> MLHLSAAPPAPPPEVTATARPCLCSVGRRGDGGKMAAAGALERSFVELSGAERERPRHFREFTVCSIGTANAVAGAVKYSESAGGFYYVESGKLFSVTRNRFIHWKTSGDTLELMEESLDINLLNNAIRLKFQNCSVLPGGVYVSETQNRVIILMLTNQTVHRLLLPHPSRMYRSELVVDSQMQSIFTDIGKVDFTDPCNYQLIPAVPGISPNSTASTAWLSSDGEALFALPCASGGIFVLKLPPYDIPGMVSVVELKQSSVMQRLLTGWMPTAIRGDQSPSDRPLSLAVHCVEHDAFIFALCQDHKLRMWSYKEQMCLMVADMLEYVPVKKDLRLTAGTGHKLRLAYSPTMGLYLGIYMHAPKRGQFCIFQLVSTESNRYSLDHISSLFTSQETLIDFALTSTDIWALWHDAENQTVVKYINFEHNVAGQWNPVFMQPLPEEEIVIRDDQDPREMYLQSLFTPGQFTNEALCKALQIFCRGTERNLDLSWSELKKEVTLAVENELQGSVTEYEFSQEEFRNLQQEFWCKFYACCLQYQEALSHPLALHLNPHTNMVCLLKKGYLSFLIPSSLVDHLYLLPYENLLTEDETTISDDVDIARDVICLIKCLRLIEESVTVDMSVIMEMSCYNLQSPEKAAEQILEDMITIDVENVMEDICSKLQEIRNPIHAIGLLIREMDYETEVEMEKGFNPAQPLNIRMNLTQLYGSNTAGYIVCRGVHKIASTRFLICRDLLILQQLLMRLGDAVIWGTGQLFQAQQDLLHRTAPLLLSYYLIKWGSECLATDVPLDTLESNLQHLSVLELTDSGALMANRFVSSPQTIVELFFQEVARKHIISHLFSQ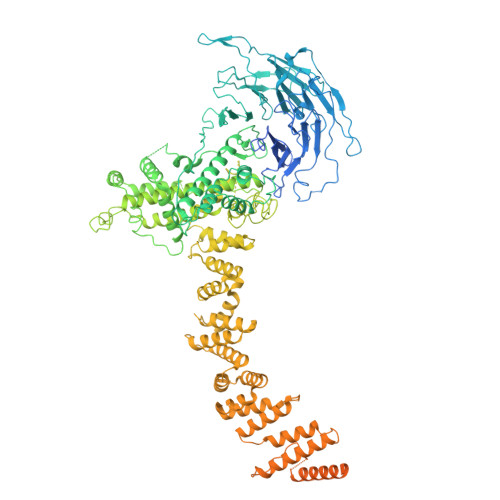PKAPLSQTGLNWPEMITAITSYLLQLLWPSNPGCLFLECLMGNCQYVQLQDYIQLLHPWCQVNVGSCRFMLGRCYLVTGEGQKALECFCQAASEVGKEEFLDRLIRSEDGEIVSTPRLQYYDKVLRLLDVIGLPELVIQLATSAITEAGDDWKSQATLRTCIFKHHLDLGHNSQAYEALTQIPDSSRQLDCLRQLVVVLCERSQLQDLVEFPYVNLHNEVVGIIESRARAVDLMTHNYYELLYAFHIYRHNYRKAGTVMFEYGMRLGREVRTLRGLEKQGNCYLAALNCLRLIRPEYAWIVQPVSGAVYDRPGASPKRNHDGECTAAPTNRQIEILELEDLEKECSLARIRLTLAQHDPSAVAVAGSSSAEEMVTLLVQAGLFDTAISLCQTFKLPLTPVFEGLAFKCIKLQFGGEAAQAEAWAWLAANQLSSVITTKESSATDEAWRLLSTYLERYKVQNNLYHHCVINKLLSHGVPLPNWLINSYKKVDAAELLRLYLNYDLLEEAVDLVSEYVDAVLGKGHQYFGIEFPLSATAPMVWLPYSSIDQLLQALGENSANSHNIALSQKILDKLEDYQQKVDKATRDLLYRRTL>[4x]MHHHHHHHHENLYFQGSSSQEKNGKGEVIIPKEKFWKISTPPEAYWNREQEKLNRQYNPILSMLTNQTGEAGRLSNISHLNYCEPDLRVTSVVTGFNNLPDRFKDFLLYLRCRNYSLLIDQPDKCAKKPFLLLA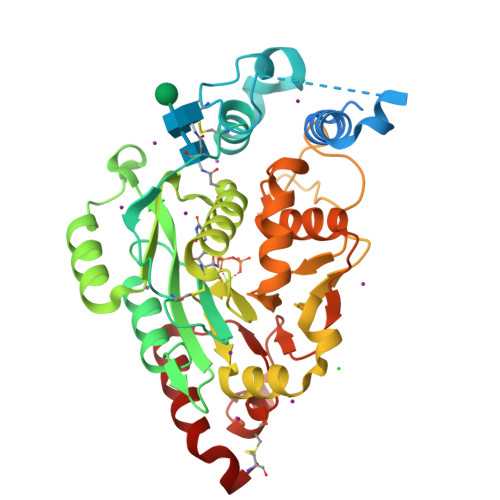IKSLTPHFARRQAIRESWGQESNAGNQTVVRVFLLGQTPPEDNHPDLSDMLKFESEKHQDILMWNYRDTFFNLSLKEVLFLRWVSTSCPDTEFVFKGDDDVFVNTHHILNYLNSLSKTKAKDLFIGDVIHNAGPHRDKKLKYYIPEVVYSGLYPPYAGGGGFLYSGHLALRLYHITDQVHLYPIDDVYTGMCLQKLGLVPEKHKGFRTFDIEEKNKNNICSYVDLMLVHSRKPQEMIDIWSQLQSAHLKC P-HYDROXYBENZOIC ACID | C7 H6 O3 | 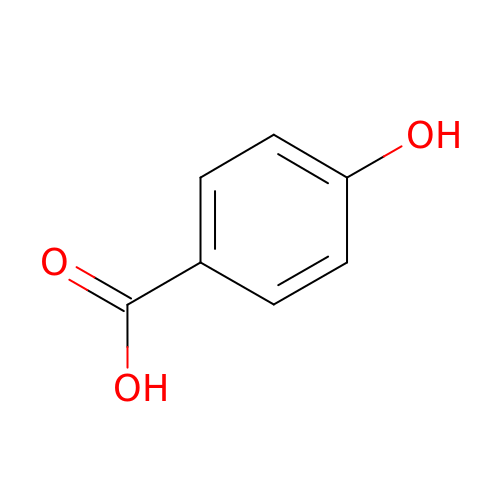FJKROLUGYXJWQN-UHFFFAOYSA-N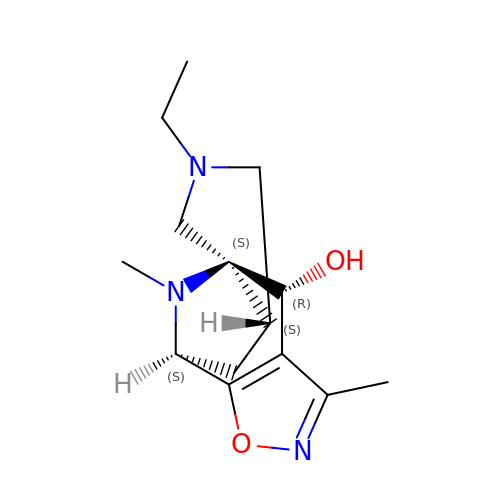(4R,4aS,7aS,9S)-6-ethyl-3,10-dimethyl-5,6,7,7a,8,9-hexahydro-4H-4a,9-epiminopyrrolo[3',4':5,6]cyclohepta[1,2-d][1,2]oxazol-4-ol | C14 H21 N3 O2 | BZPBUUKNGNRKPU-DUBDDPSESA-N>MGRIKNKQFAVIGLGRFGGSICKELHRMGHEVLAVDINEEKVNAYASYATHAVIANATEENELLSLGIRNFEYVIVAIGPNIQASTLTTLLLKELDIP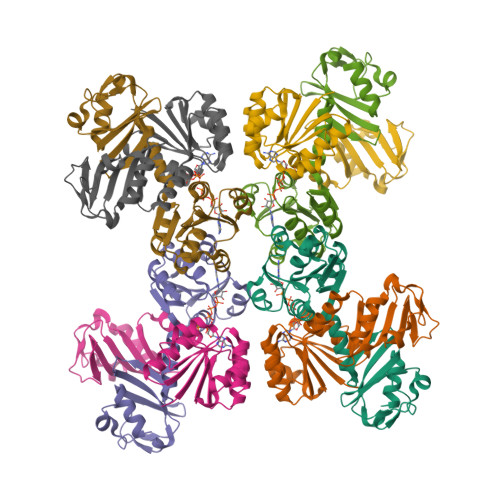NIWVKAQNYYHHKVLEKIGADRIIHPEKDMGVKIAQSLSDENVLNYIDLSDEYSIVELLATRKLDSKSIIDLNVRAKYGCTILAIKHHGDICLSPAPEDIIREQDCLVIMGHKKDIKRFENEGM[8x]>MRLLAVFVSSRLSPEDPLYARWVRYGEVLAEEGFGLACGGYQGGMEALARGVKAKGGLVVGVTAPAFFPERRGPNPFVDLELPAATLPQRIGRLLDLGAGYLALPGGVGTLAELVLAWNLLYLRRGVGRPLAVDPYWLGLLKAHGEIAPEDVGLLRVVADEEDLR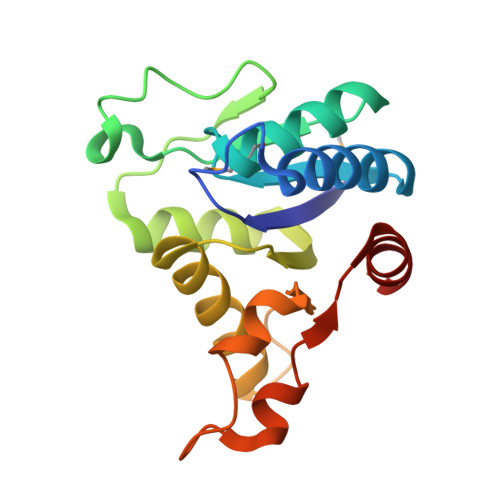RFLRSL[2x]(4aR,7aR,9R)-3,4,7,7a,8,9-hexahydro-4a,9-epoxypyrrolo[3',4':4,5]cyclohepta[1,2-d]imidazole-6(5H)-carbaldehyde 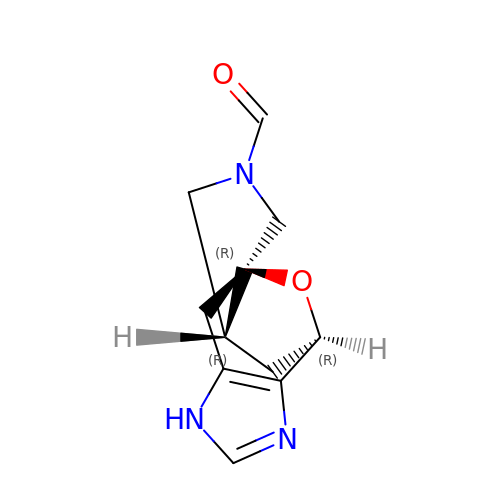| C11 H13 N3 O2 | XRNLVBAEYBLIIG-ZOFUNIGCSA-N>[12x]MDKFRVQGPTKLQGEVTISGAKNAALPILFAALLAEEPVEIQNVPKLKDVDTSMKLLSQLGAKVERDGSVHIDARDVNVFCAPYDLVKTMRASIWALGPLVARFGQGQVSLPGGCTIGARPVDLHISGLEQLGATIKLEEGYVKASVDGRLKGAHIVMDKVSVGATVTIMCA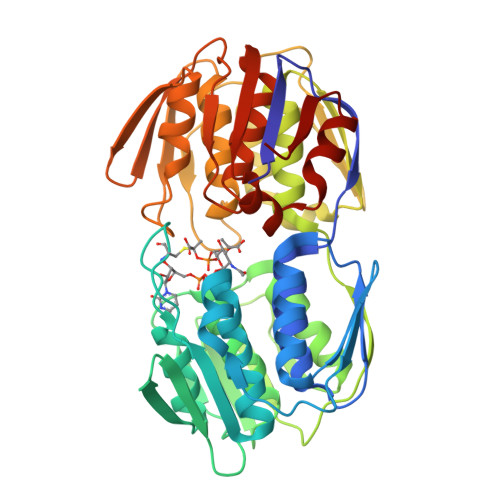ATLAEGTTIIENAAREPEIVDTANFLITLGAKISGQGTDRIVIEGVERLGGGVYRVLPDRIETGTFLVAAAISRGKIICRNAQPDTLDAVLAKLRDAGADIEVGEDWISLDMHGKRPKAVNVRTAPHPAFPTDMQAQFTLLNLVAEGTGFITETVFENRFMHVPELSRMGAHAEIESNTVICHGVEKLSGAQVMATDLRASASLVLAGCIAEGTTVVDRIYHIDRGYERIEDKLRALGANIERVKG> KTSDANETEDHLESLICKVGEKSACSLESNLEGLAGVLEADLPNYKSKILRLLCTVARLLPEKLTIYTTLVGLLNARNYNFGGEFVEAMIRQLKESLKANNYNEAVYLVRFLSDLVNCHVIAAPSMVAMFENFVSVTQEEDVPQVRRDWYVYAFLSSLPWVGKELYEKKDAEMDRIFANTESYLKRRQKTHVPM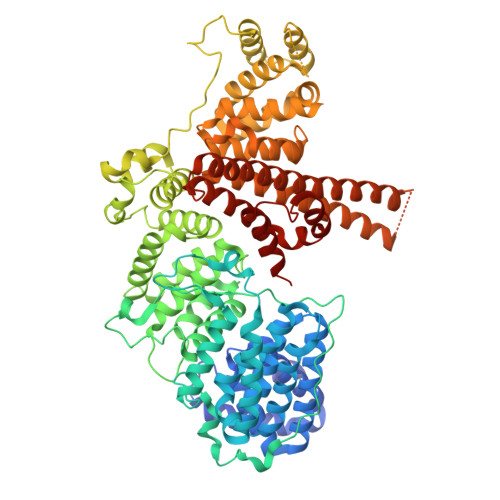LQVWTADKPHPQEEYLDCLWAQIQKLKKDRWQERHILRPYLAFDSILCEALQHNLPPFTPPPHTEDSVYPMPRVIFRMFDYTDDPEGPVMPGSHSVERFVIEENLHCIIKSHWKERKTCAAQLVSYPGKNKIPLNYHIVEVIFAELFQLPAPPHIDVMYTTLLIELCKLQPGSLPQVLAQATEMLYMRLDTMNTTCVDRFINWFSHHLSNFQFRWSWEDWSDCLSQDPESPKPKFVREVLEKCMRLSYHQRILDIVPPTFSALCPSNPTCIYKYGDESSNSLPGHSVALCLAVAFKSKATNDEIFSILKDVPNPNQDDDDDEGFSFNPLKIEVFVQTLLHLAAKSFSHSFSALAKFHEVFKTLAESDEGKLHVLRVMFEVWRNHPQMIAVLVDKMIRTQIVDCAAVANWIFSSELSRDFTRLFVWEILHSTIRKMNKHVLKIQKELEEAKEKLARQHDGVLEEQIERLQEKVESAQSEQKNLFLVIFQRFIMILTEHLVRCETDGTSVLTPWYKNCIERLQQIFLQHHQIIQQYMVTLENLLFTAELDPHILAVFQQFCALQA> KRLSSHHAIVCGAASATAASTRFGDVVGGGSSCTATSPLFAAQRGRFYRPLVNQGINLWRSRMGRLHKGWTTWEYNRDVIPDPRPFPEPAVNNYFGRSRIWNPIAGKIGLVNRKAEEWGWPHQRPPPTGLRRSPEYFPFFFSRYFPDVEVRLVLDSVLNNETTRPIFHIPQDMSKQELVNYLKNIYNIDNVVRI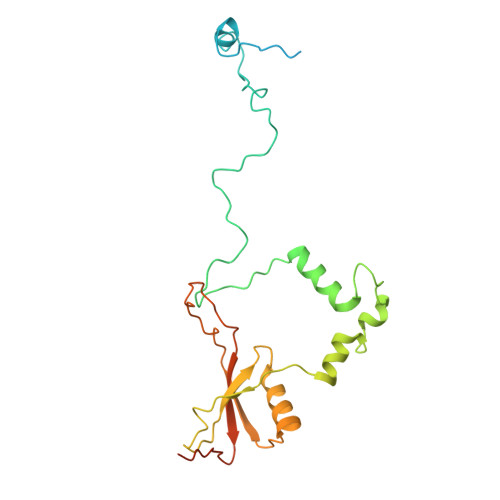RVRNMRGRRFKNEVGEIKSLPDYKVAVVELDSPVSIVFKQIKGTEDTPDNKPAAQIT3-(4-fluorophenyl)-4-(imidazol-1-ylmethyl)-1-phenyl-pyrazole 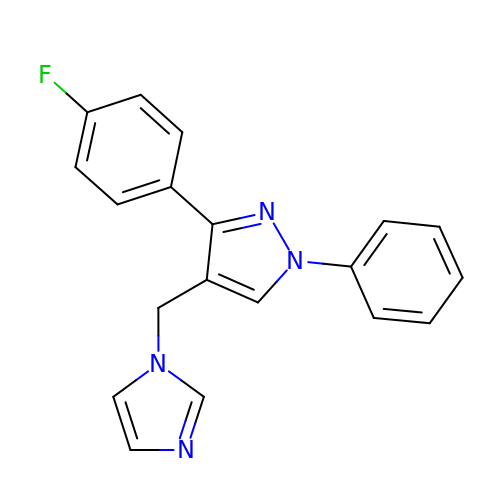| C19 H15 F N4 | KWPMFVYWNXVKNC-UHFFFAOYSA-N The three largest gene segments of the Thogotoviruses, THOV, DHOV and JOSV are homologous to those of IAV and code for the heterotrimeric polymerase. In this paper we present the atomic structures of the putative PB2 cap binding and 627 domains of THOV and the putative PA N-terminal endonuclease domains of THOV and DHOV. Despite very low sequence homologies, all domains have similar folds to those of the corresponding IAV polymerase domains. However, the critical active site residues in the putative cap binding and endonuclease domains are not conserved in THOV and DHOV and, contrary to the case of IAV polymerase, neither domain shows the expected in vitro biochemical activity.

To overcome this problem, we produced the homologous domain from DHOV PA (40% identity between full-length THOV and DHOV PA, 29% for the N-terminal part), which readily crystallized and the structure was solved by the Single wavelength Anomalous Dispersion (SAD) method using seleno-methionine labelled protein. The resultant model was then used to solve the THOV PA-Nter structure by molecular replacement. The three domains clearly have the same fold, and THOV and DHOV PA-Nter are very similar. For THOV and DHOV PA-Nter the putative active site is more like an extended groove and furthermore, is positively charged. Indeed of the cation binding residues, only an equivalent of influenza Asp108 (PD motif) is found in THOV and DHOV PA-Nter, respectively Asp-86 and Asp-87. The extra positive charge in the putative active sites of THOV and DHOV PA-Nter arises from the replacement of acidic residues and the introduction of extra lysines (Lys38, Lys61 and Lys97 for THOV and Lys39 and Lys100 for DHOV PA-Nter). Using the Thermofluor assay to measure apparent melting temperature (Tm), we found that in the absence of any divalent cations, the Tm of THOV and DHOV PA-Nter domains were respectively 41 and 53°C compared with 44°C for IAV. For the DHOV domain, which is already more stable, addition of these ions has little effect, giving no indication of cation binding. Finally, neither THOV nor DHOV PA-Nter show any nuclease activity against various RNAs under conditions where IAV PA-Nter does. Our structural and biochemical results therefore strongly suggest that THOV and DHOV PA-Nter domains neither bind divalent cations nor are active endonucleases.

>[2x]GAMDRHKPKSISSEIWALSETSKEWMSNLRPLEARIVECIKYTVCCHISDMHLHNGVPRYIVNMWTPPEVADQEMKRQNLIFARPNVPDLLDLKERKGVYVKVYPDNGTPTDYQTAENEIFVRVSLSGQMSPITREYLDEVQRQDVTNFLVTIYNESLESNLLERMQELYDTD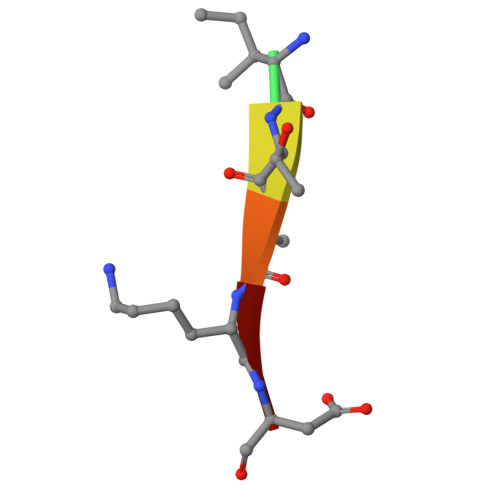> XITAKD>[2x]GPGFDYAVAMAKRNIVTATTSKGEFTMLGVHDNVAILPTHASPGESIVIDGKEVEILDAKALEDQAGTNLEITIITLKRNEKFRDIRPHIPTQITETNDGVLIVNT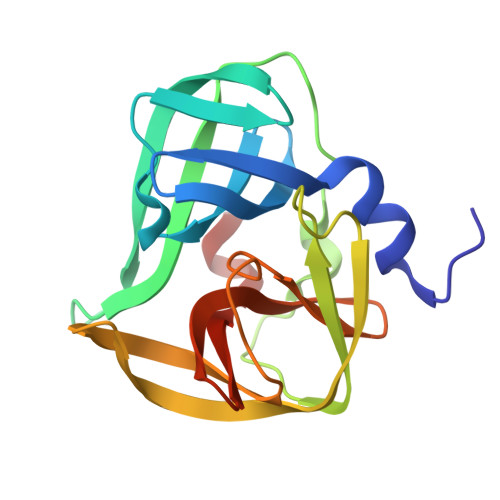SKYPNMYVPVGAVTEQGYLNLGGRQTARTLMYNFPTRAGQCGGVITCTGKVIGMHVGGNGSHGFAAALKRSYFTQSQ> MTVPDEPVGFWVESIPGNDHTLLLTWSETKGAKYYEIYLVSDSTYKFIASTDKLEYYVTNLSP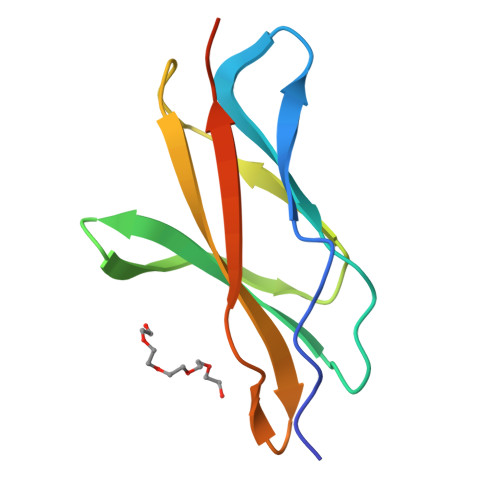NTKYTFALIAVNELGPSNFVTASSTTDRGGHHHHHH>TRDQNGTWEMESNENFEGYMKALDIDFATRKIAVRLTQTLVIDQDGDNFKTKCTSTFRNYDVDFTVGVEFDEYTKSLDNRHVKALVTWEGDVLVCVQKGEKENRGWKKWIEGDKLYLELTCGDQVCRQV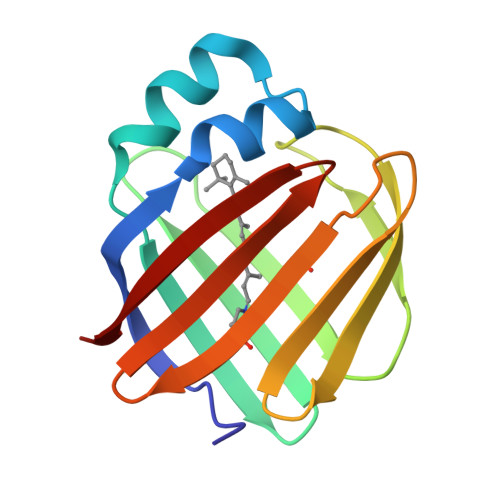FKKK[2x]>SIEKIWAREILDSRGNPTVEVDLYTAKGLFRAAVPSGASTGIYEALELRDGDKQRYLGKGVLKAVDHINSTIAPALISSGLSVVEQEKLDNLMLELDGTENKSKFGANAILGVSLAVCKAGAAERELPLYRHIAQLAGNSDLILPVPAFNVINGGSHAGNKLAMQEFMILPVGAESFRDAMRLGAEVYHTLKGVIKDKYGKDATNVGDEGGFAPNILENSEALELVKEAIDKAGYTEKIVIGMDVAASEFYRDGKYDLDFKSPTDPSRYITGDQLGALYQDFVRDYPVVSIEDPFDQDDWAAWSKFTANVGIQIVGDDLTVTNPKRIERAVEEKACNCLLLKVNQIGSVTEAIQACKLAQENGWGVMVSHRSGETEDTFIADLVVGLCTGQIKTGAPCRSERLAKYNQLMRIEEELGDEARFAGHNFRNPS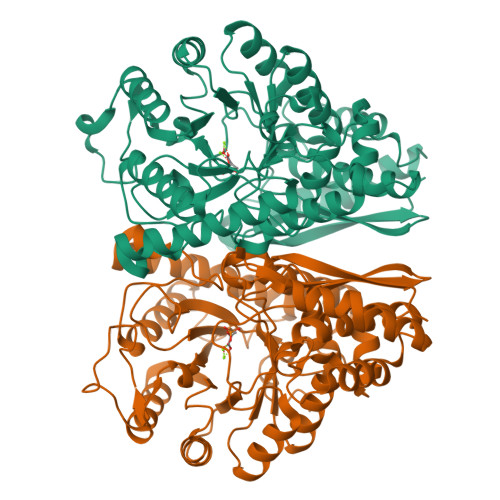VLHHHHHHHHHH[2x]>[2x]MENSFKAALKAGRPQIG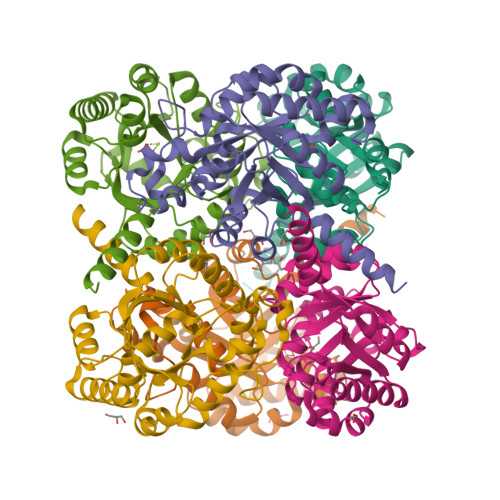LWLGLSSSYSAELLAGAGFDWLLIDGEHAPNNVQTVLTQLQAIAPYPSQPVVRPSWNDPVQIKQLLDVGTQTLLVPMVQNADEAREAVRATRYPPAGIRGVGSALARASRWNRIPDYLQKANDQMCVLVQIETREAMKNLPQILDVEGVDGVFIGPADLSADMGYAGNPQHPEVQAAIEQAIVQIRESGKAPGILIANEQLAKRYLELGALFVAVGVDTTLLARAAEALAARFG>[2x]PPESDGFSDVRKVGYLRKPKSMHKRFFVLRAASEAGGPARLEYYENEKKWRHKSSAPKRSIPLESCFNINKRADSKNKHLVALYTRDEHFAIAADSEAEQDSWYQALLQLHNRAKGHHDGA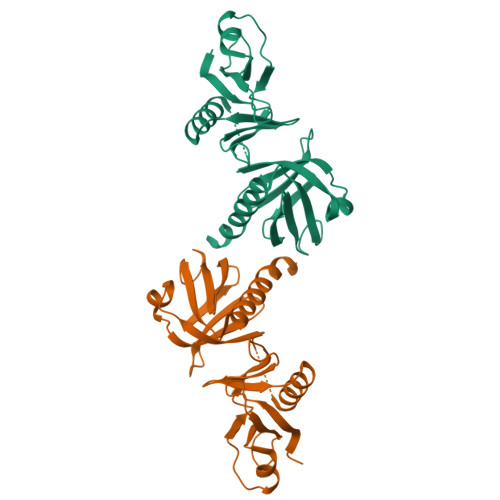AALGAGGGGGSCSGSSGLGEAGEDLSYGDVPPGPAFKEVWQVILKPKGLGQTKNLIGIYRLCLTSKTISFVKLNSEAAAVVLQLMNIRRCGHSENFFFIEVGRSAVTGPGEFWMQVDDSVVAQNMHETILEAMRAMSDEFRPR>[8x]KNSLPYGKINGTYKGTEKEKIKFSSEGSFDPDGKIVSYEWDFGDGNKSNEENPEHSYDKVGTYTVKLKVTDDKGESSVSTTTAEIKD

Clostridium histolyticum collagenases ColG and ColH are segmental enzymes that are thought to be activated by Ca2+-triggered domain reorientation to cause extensive tissue destruction. The collagenases consist of a collagenase module (s1), a variable number of polycystic kidney disease-like (PKD-like) domains (s2a and s2b in ColH and s2 in ColG) and a variable number of collagen-binding domains (s3 in ColH and s3a and s3b in ColG). The X-ray crystal structures of Ca2+-bound holo s2a (space group C2), Ca2+-free apo s2a (space group P61), Ca2+-bound holo s2b (space group P21) and two new forms of N-terminally truncated wild-type apo s2 (space groups P21 and P212121) are reported for the first time. Comparison of crystal structures of ColG s2 with crystal structures of ColH s2a and s2b suggests that despite common tertiary folds, PKD-like domains can be grouped into two subsets.

The eight holo s2a molecules are virtually identical (average r.m.s.d. of 0.2 ± 0.1 Å). Here, the molecules spiral along the crystallographic axis. Along this axis, molecule pairs A and G, B and E, C and F, and D and H are related by NCS translation that results in an off-origin peak that is 63.9% of the origin peak in the Patterson map. The holo and apo structures resemble each other (r.m.s.d. = 0.6 ± 0.2 Å). As expected, the most notable difference between the structures occurs near the N-terminus, where Ca2+ reorients the interacting residues Asn685 and Ser686. One calcium-binding site with a pentagonal bipyramidal geometry was identified near the N-terminus in each domain. The pentagonal base is composed of OD1 of Asn685, the main-chain carbonyl of Ser686, OD1 and OD2 of Asp713 and a water molecule, while the axial positions are filled by OD1 of Asp715 and OD2 of Asp754. Unlike s2b or s2, s2a truncates β-strand A through an approximately 126° rotation of the ψ bond of Ile692. In the s2a structures the termini are the most flexible. As mentioned, the B-factor trends in all holo and apo s2a structures are similar despite the difference in crystal packing.>[4x]GSAMDPGSGSGNSHNSLMKLLLLNGHGINMHVDGAKLHIKDGRFSTTEEPQEYVFSPKRIDIDGIIIYGKSGNLTLEAIRWLIKHNVQVSILDWNGKLLTTMLPPESTNLRTKFAQYHAFEDKEARLEIAKKFIEAKFYKSKAVLDFLSQRYPEINFDILDGLTKLKDVKSTREILGVEGTLAGKYWIEFSKAVPKEYDFSNRIDQFRRAMGSGDMINTMLNYGYSLLEAECLKAINSVGLDTHVGFLHEMAPSKNSLAYDLQEPFRFIVDLAVISLIESGAMESKDFIRTENYNLRLKPTGARKIVNEFSNTLNKKVSYQGKESTWSYVIFLKVRELAHYLTSKKEKLDFTKPEYEIERIDSYDIRQKILSISYVDWKKLGFSKGTLHYMKQNAKSDKPFTLNAHVLERVNKWEALVSSQRDGRENLYFQ

Phylogenetic analysis of Cas1 proteins suggests that they may have originated from casposons, a novel class of putative DNA transposons in which a Cas1 homolog (the ‘casposase’) functions as the transposase (Krupovic et al., 2014; Koonin and Makarova, 2017). To understand how Cas1 of CRISPR-Cas systems may have evolved from a transposase, we have characterized the biochemical properties of a casposase from Methanosarcina mazei. We have also determined its three-dimensional structure bound to branched DNA that represents the product of casposon end insertion into a specific sequence at the 3'-end of a host tRNA-Leu gene. We show that the casposase is tetrameric when bound to its target site and can site-specifically integrate a range of substrates including casposon ends with 3'-overhangs and even short single-stranded DNA ends as well as ssRNA.

The pseudo two-fold symmetric complex is a clamp-like tetramer in which two casposase dimers hold the double-stranded target site between them, with the 5' termini of the single-stranded casposon ends emerging through a narrow slot in the bottom of the clamp. Each casposase monomer exhibits the fold expected of a Cas1 homolog (Wiedenheft et al., 2009; Figure 5—figure supplements 2 and 3), with a canonical eight-stranded N-terminal domain and a globular catalytic domain that brings conserved active site residues (E162, H232, E247) into close proximity. In the integration product complex, each dimer is functionally and structurally asymmetric with a ‘catalytic’ monomer whose active site contains the scissile phosphate group that links transposon end DNA and the target site, and a ‘noncatalytic’ monomer in which the active site is located on the periphery of the assembly facing away from the DNA. In the tetrameric complex with the integration product DNA, we observe two dimer-to-dimer interactions formed by the convergence of helix α1 (residues 59–67) and a loop (residues 39–44 between β4 and β5) from each noncatalytic monomer with two loops (residues 182–199 and 275–278) from the opposing catalytic monomer. In the casposase complex structure, the total casposase-dsDNA interface buries ~4700 Å2 of solvent-accessible surface but only two specific contacts mediate the interaction with the target DNA: between R191 and G22 (i.e., the base opposite the first C of the 5'-CGCA motif) and between R192 and G20 (the base opposite the second C of the 5'-CGCA motif). The bound target in the integration product complex is almost perfectly straight B-form DNA, unlike the severely bent targets observed in other DNA transpososomes and retroviral intasomes (for example, Montaño et al., 2012; Maertens et al., 2010). Although the only base-specific interaction is between the first C of the casposon DNA (C8) and the side chain of K238, several residues interact with the phosphate backbone (H232, R250, Y206, R280, and R287) and there are arrays of stacking interactions.>SDRAMMNAFKEITTMADRINLPRNIVDRTNNLFKQVYEQKSLKGRANDAIASACLYIACRQEGVPRTFKEICAVSRISKKEIGRCFKLILKALETSVDLITTGDFMSRFCSNLCLPKQVQMAATHIARKAVELDLVPGRSPISVAAAAIYMASQASAEKRTQKEIGDIAGVADVTIRQSYRLIYPRAPDLFPTDFKFDTPVDKLPQL[5x];>GSGIVPQLQNIVSTVNLGCKLDLKTIALRARNAEYNPKRFAAVIMRIREPRTTALIFSSGKMVCTGAKSEEQSRLAARKYARVVQKLGFPAKFLDFKIQNMVGSCDVKFPIRLEGLVLTHQQFSSYEPELFPGLIYRMIKPRIVLLIFVSGKV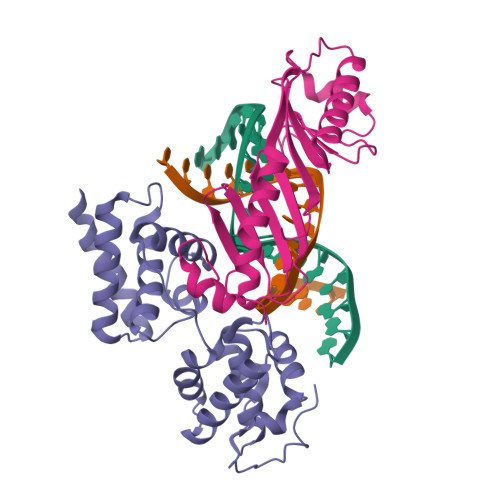VLTGAKVRAEIYEAFENIYPILKGFRK[5x]> SMKDVPDSQQHPAPEKSSKVSEQLKCCSGILKEMFAKKHAAYAWPF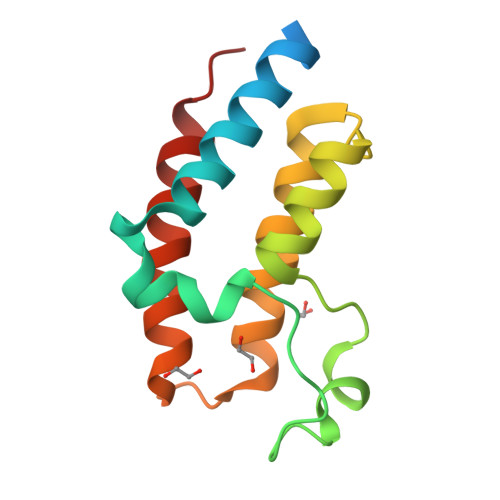YKPVDVEALGLHDYCDIIKHPMDMSTIKSKLEAREYRDAQEFGADVRLMFSNCYKYNPPDHEVVAMARKLQDVFEMRFAKMPDE> VRLPGLAAMRQGTRLFTPEQGEDLREALRRRRGSFQTTCEVTSETTFAAARRLREKASALAALNFASAKNPGGGFLGGAQAQEEDLCRGSGLYFSLTSPQAEPYYAVNRQSHSALYTDHLIYSPQVPIFRDDAGQLLPAPVPVNIITAPAPNAGAVAQSRPEQLPQVLPTLRERARRVLGVAAWMEQTHLVLGAWGCGVFRNDPAGVARTFRELLEGEAQGAFEHVTFAVLDNHPQHPRLGAFRRELESLC

Despite the abundance of PARP1, most of the PAR generated by DNA damage is rapidly degraded, with a half-life of less than 1 min by poly (ADP-ribose) glycohydrolase (PARG). The radio-resistant bacterium D. radiodurans encodes a PARG homolog, DrPARG, whose expression is upregulated after radiation damage, so it might play an important role in DNA repair. Our study demonstrates that DrPARG is involved in catalyzing the breakdown of endogenous PAR and DNA repair in D. radiodurans. From observing the structural peculiarities of DrPARG, we show that although previously thought to be an obligate exo-glycohydrolase, bacterial PARG could exert both exo- and endo-glycohydrolase functions.

To clarify the effect of Thr267 on enzyme activity of DrPARG, we generated mutants of DrPARG by substituting Thr267 for arginine or lysine. Furthermore, we determined crystal structures of DrPARG T267R and T267K in complex with ADP-ribose for understanding the detailed interactions. The crystal structures of T267R and T267K belonged to the space group P3221. In consistent to the secondary structure analyzed by CD spectrum, the substitution of the residue did not cause dramatic alterations to overall structure compared with the wild-type enzyme with root mean square deviation to wild type of 0.50 and 0.43 Å for T267R and T267K, respectively. As compared with the ADP-ribose bound TcPARG structure, the side-chain position of Arg267 was fixed like that of TcPARG by regaining complex hydrogen bonding with ADP-ribose and neighboring His262 and Cys225 as well as ionic interaction with Asp260, which suggested that the endo-glycohydrolase activity was impaired. Compared with the solvent-accessible 2′-OH with n + 1 linkage point observed in wild-type, which were inaccessible and less accessible to solvent in the complex structures of T267R and T267K, respectively. PARG cleavage assay in vitro showed T267R and T267K mutants with decreased hydrolysis PAR activity as compared with the wild-type enzyme. Consistent with in vitro cleavage assay, the mutants designed for blocking endo-glycohydrolase activity showed significantly decreased turnover rate Kcat as compared with the wild-type DrPARG, so the mutants may have reduced activity toward PAR. Short-chain PAR was not detected in the filtrates of the two DrPARG mutants T267R and T267K, as well as the TcPARG, although the mutants still hydrolyzed PAR. Since T267R and T267K DrPARG catalyze the hydrolysis of PAR without generating short-chain PAR but oligo ADP-ribose, the establishment of endo-glycohydrolase activity was not solely accounted from the lack of steric hinderance near 2′-OH.> MRLTKFTDLALRSLMRLAVVRDGDEPLATREVAEVVGVPYTHAAKAITRLQHLGVVEARRGRGGGLTLTDLGRRVSVGWLVRELEGEAEVVDCEGDNPCPLRGACRLRRALRDAQEAFYAALDPLTVTDLVAAPTGPV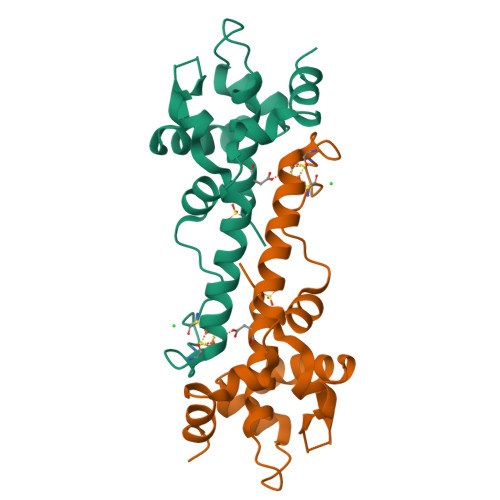LLGLTDRPSGKLAAALEHHHHHH>ETGESLAKETAFVEVVLFESSPNGDYKTHTTELQGRFSRAGATISAEGEIVQMHPLGLCNNNDEEDLYEYGWVGVVKLEQPEMDPKPCLTVLGKAKRAVQRGATAVIFDVSDNPDAVEQLNQGLEDPLKRPVVYMKGMDAIKLMNIVNKQKGARARIQHRPPRQPTEYFDGTHHHHHHHHHH[2x]

Rspo (R-spondin, also roof plate-specific spondin) proteins are evolutionarily conserved from fish to humans and have well-documented roles in a broad range of developmental and physiological processes resulting from enhancement of canonical and non-canonical Wnt signalling. ZNRF3/RNF43 specifically targets these Wnt receptors for ubiquitination and turnover, hence reducing Wnt signalling responses. Direct extracellular interaction with Rspo proteins inhibits ZNRF3/RNF43 activity. Here we report a molecular level analysis of the ZNRF3/RNF43 ectodomain structure and its interactions with Rspo proteins.

By using a combination of heavy atom and molecular-replacement-based phasing strategies, we determined multiple crystal structures for Xenopus (x) Rspo2Fu1–Fu2 (highest resolution 2.2 Å), xZNRF3ecto, zebrafish (z) ZNRF3ecto and mouse (m) ZNRF3ecto, (highest resolutions 2.4, 1.6 and 2.0 Å, respectively), plus complexes comprising xZNRF3ecto–xRspo2Fu1–Fu2, mZNRF3ecto–mRspo2Fu1–Fu2, mZNRF3ecto–xRspo2Fu1–Fu2 and xRNF4F3ecto–xRspo2Fu1–Fu2 (at 2.1, 2.8, 2.4 and 2.7 Å, respectively). The ZNRF3ecto crystal structures revealed a distinctive variant of the protease-associated domain topology. Two β-sheets (comprising β2, β1, β7, β3 and β4, β5, β6 strands, respectively) splay apart, accommodating an α-helix (αC) at the open edge; two additional α-helices (αA and αB) pack against the β4, β5 and β6 face of this distorted β-sandwich. A disulphide bridge, conserved across species, links two structurally elaborate loops, β3–β4 and β4–αA. The resultant single-domain structure is relatively compact. The crystal structures for apo xZNRF3ecto, zZNRF3ecto and mZNRF3ecto showed no major differences in the main chain conformation. Comparisons of ZNRF3ecto structures for proteins crystallized in several different crystal lattices, or for crystals containing multiple copies in the asymmetric unit, consistently highlighted an acidic region (N105-E114; residue numbering is for mouse sequences unless otherwise stated) within the β3–β4 loop, the short αC–β7 loop and the extended β1–β2 hairpin as flexible elements of the fold. All but two of these crystal structures reveal an extensive interface (average interface area 992±109 Å2) formed between two ZNRF3ecto polypeptide chains. The interaction is twofold symmetric; strands β3 and β7 of the ‘subunits’ abut face-to-face at the core of the dimer. The β1–β2 hairpin forms a second interface by reaching out to embrace helix αA and the β3–β4 loop in the opposing subunit.> MILLDTNVISEPLRPQPNERVVAWLDSLILEDVYLSAITVAEMRLGVALLLNGKKK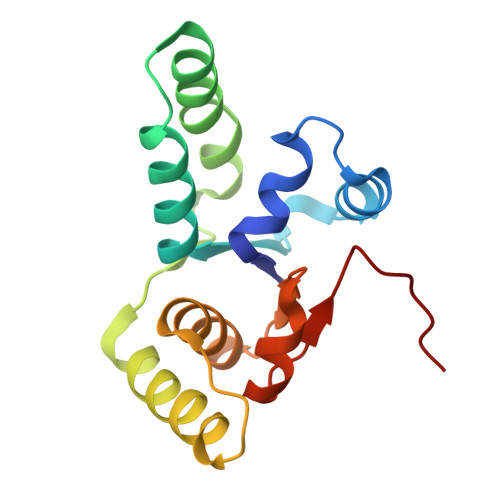NVLHERMEQSILPLFAGRILPFDEPVAAIYAQIRSYAKTHGKEIAAADGYIAATAKQHSMTVATRDTGSFFAADVAVFNPWHLEHHH N-ETHYLMALEIMIDE | C6 H7 N O2 | 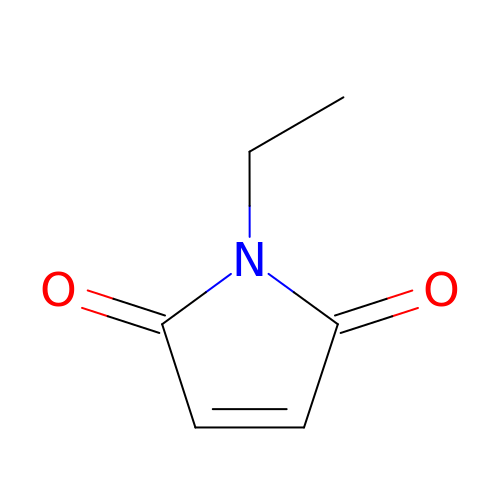HDFGOPSGAURCEO-UHFFFAOYSA-N> MSQLWVLYETYCQLFSLTNEEKVI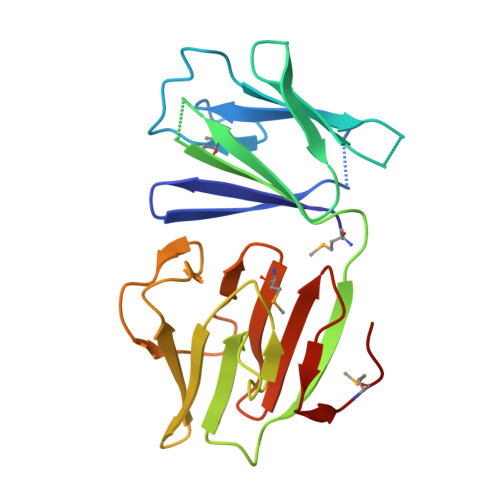VIGNQLEHHVTVSSFSFRNGYIQIEKKSDGSTLAVLQGGRQIGELKPRCSITIDVDGQQMTIAWSGEEQRKYVYYVGQQSEVLVSNDPQADIETTNARFSLRKHRGQWVVIPDDDAPLFLNGVQLSDAVSLRNGDVLLCPYMQFVFIEEDLLAVTSSEEVVSSLTETMPPLS>[2x]SNAY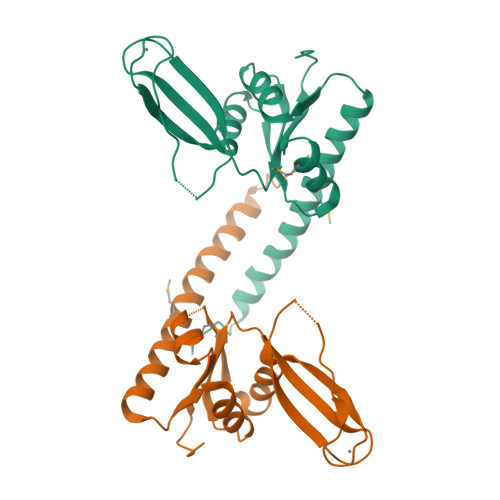TDESGLSELVNAAGEKLQDLELMGQKNAVRDFFKELIADSGKVAYGESQVRANLEINSVDVLLLSEDLRAERVTTKCSVCGYENKWTRRWKPGEPAPAAGNCPKCGSSLEVTDVTDIVDEFSELADKSNAKVVFVSTDFDEGSQLMNAFGGIAAILRYNTGV> MYATMESVRLQSEAQQLAEMILQSETAENYRNCYKRLQEDEEAGRIIRSFIKIKEQYEDVQRFGKYHPDYREISRKMREIKRELDLNDKVADFKRAENELQSILDEVSVEIGTAVSEHVKV;> GPMTLYSKKDIVQQARNLAKMISETEEVDFFKRAEAQINENDKVSTIVNQIKALQKQAVNLKHYEKHEALKQVEAKIDALQEELEEIPVIQEFRDSQMEVNDLLQLVAHTISNQVTNEIITSTG

In Bacillus subtilis, the RicA (YmcA), RicF (YlbF), and RicT (YaaT) proteins accelerate the phosphorylation of the transcription factor Spo0A, contributing to genetic competence, sporulation, and biofilm formation, and are also essential for the correct maturation of several protein-encoding and riboswitch RNAs. These proteins form a stable complex (RicAFT) that carries two [4Fe-4S]+2 clusters. We show here that the complex is a 1:1:1 heterotrimer, and we present the X-ray crystal structures of a RicAF heterotetramer and of a RicA dimer.

Despite the fact that RicA and RicF have only about 20% sequence identity, their monomeric structures as well as the structures of RicA and RicAF are nearly identical. In fact, superposition of RicA dimer and of RicAF revealed a root mean square deviation (RMSD) value for 166 aligned Cα of 0.982 Å. The most poorly aligned portions of these structures occurred in the α3-α4 flaps, suggesting that there may be some flexibility in the turns connecting α3 to α4 and α4 to α5. We note that the gap separating the RicA and RicF flaps is relatively large (∼50 Å), and we speculate that RicT may occupy this space in the RicAFT complex. Despite the structural similarity of RicA and RicAF, the SEC results suggest the RicAF forms a higher-order oligomer. Consistent with the RicAF SEC results, we identified a RicAF crystallographic tetramer. Thus, we tentatively conclude that RicAF is a tetramer in vitro, consisting of two molecules each of RicA and of RicF, while RicA is a homodimer. Because there is no evidence for a RicA tetramer, it would appear that the association of RicA with itself precludes tetramerization and, indeed, the tetramerization interface between RicAF dimers involves only RicA-RicF contacts (rather than RicA-RicA or RicF-RicF contacts). Examination of an equivalent construct in which 23 residues from the C-terminal tail of RicAGst were deleted similarly demonstrated a loss of association between RicAΔCF and RicT. The C termini of RicA and of RicF emerge from the RicAF structure on opposite faces of the dimer, and Fig. 7 suggests that RicT may require contact with both tails for stable association with the heterodimer. After attempted reconstitution by incubation with FeCl3 and LiS, little if any Fe above the background was detected (0.23 Fe atoms/heterodimer), indicating that this complex could not accept Fe-S clusters in the absence of RicT.>[4x]GPGSMSRQQQAQELQKQWETDPRWKGIKRAFTAEDVVRLRGSIQQEHTLAKRGAEKLWTLINNEPFVNALGALTGNQAMQQVKAGLKAIYLSGWQVAGDANVAGEMYPDQSLYPANSVPLVVKRINNTLTRADQIQWSEGKNPGDEGYVDFFAPIVADAEAGFGGVLNAFELMKAMIEAGASGVHFEDQLASVKK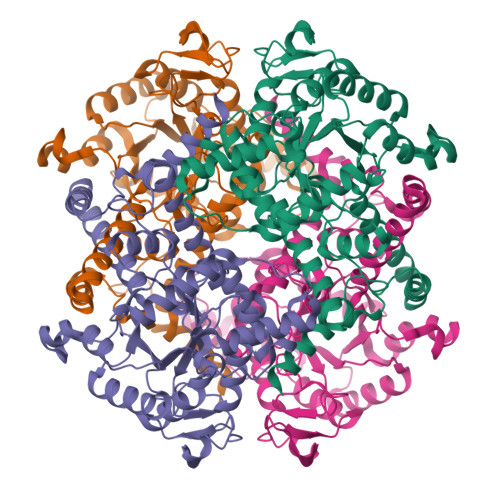CGHMGGKVLVPTREAVAKLTAARLAADVMGTPTVLVARTDAEAADLITSDIDDNDKPYLTGERTVEGFFRTKPGLEQAISRGLAYAPYADLIWCETGKPDLEYAKKFAEAIHKQFPGKLLSYNCSPSFNWKKNLDDATIAKFQKELGAMGYKFQFITLAGFHALNYSMFNLAHGYARTQMSAFVELQQAEFAAADKGFTAVKHQREVGTGYFDAVTQTVEREASTTALHGSTEDEQFFDGQKVA N-({4-[(1R)-4-(2,4-diamino-6-oxo-1,6-dihydropyrimidin-5-yl)-1-(methylsulfanyl)butyl]phenyl}carbonyl)-L-glutamic acid | C21 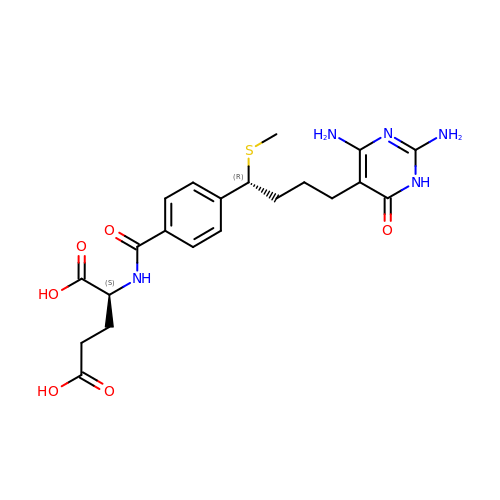H27 N5 O6 S | GEZLAVXTPLTVRU-LSDHHAIUSA-N>[2x]MAGKSPEEEHPVKAYGWAVKDRTTGILSPFKFSRRATGDNDIRIKILYCGICHTDLTSVKNEYEFLSYPLVPGMEIV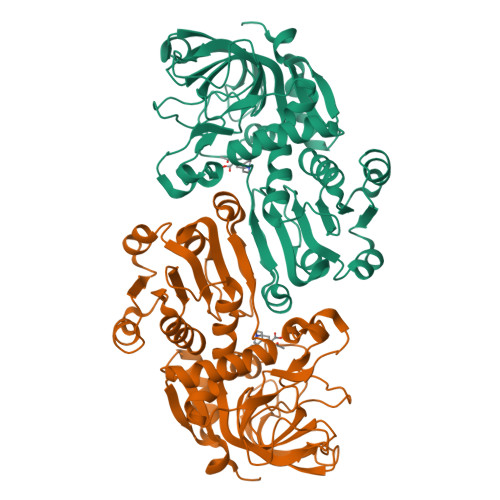GIATEVGSKVTKIKVGEKVAVAAYLGTCGKCYNCVNDLENYCPEVIIGYGTPYHDGTINYGGLSNETVVNERFVLRFPEKLSPAGGAPLLSAGITAYSAMRNHGLDKPGIHLGVVGLGGLGHLAVKFAKAFGVRVTVISTTPSKKDEAINNLGADAFLFSRDDKQMRAAIGTFDAIIDTLAVVHPIAPLLDLLRSHGKLVLVGAPSKPLELPTIPLLSGGKSLIGSAAGNVKQTQEMLDFAAEHDITANIEVIPIDYINTAMERLDKGDIRFRFVVDIENTLTPPPEP>[2x]MTHEEHHAARTLGVGKAIAVLTSGGDAQGMNAAVRAVVRVGIFTGARVFFVHEGYQGLVDGGDHIREATWESVSMMLQLGGTVIGSARCKDFREREGRLRAAHNLVKRGITNLCVIGGDGSLTGADTFRSEWSDLLSDLQKAGKITAEEATRSSYLNIVGLVGSIDNDFCGTDMTIGTDSALHRITEIVDAITTTAQSHQRTFVLEVMGRHCGYLALVTSLSCGADWVFIPECPPDDNWEDHLCRRLSETRTRGSRLNIIIVAEGAIDRNGKPITSEGVKDLVVRRLGYDTRVTVLGHVQRGGTPSAFDRILGSRMGVEAVMALLEGTPDTPACVVSLSGNQAVRLPLMECVQVTKDVTKAMDEKRFDEAMKLRGRSFMNNWEVYKLLAHIRPPAPKSGSYTVAVMNVGAPAAGMNAAVRSTVRIGLIQGNR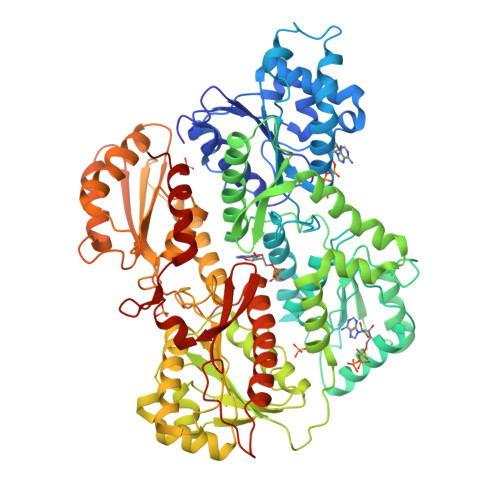VLVVHDGFEGPAKGQIEEAGWSYVGGWTGQGGSKLGSKRTLPKKSFEQISANITKFNIQGLVIIGGFEAYTGGLELMEGRKQFDELCIPFVVIPATVSNNVPGSDFSVGADTALNTICTTCDRIKQSAAGTKRRVFIIETMGGYCGYLATMAGLAAGADAAYIFEEPFTIRDLQANVEHLVQKMKTTVKRGLVLRNEKCNENYTTDFIFNLYSEEGKGIFDSRKNVLGHMQQGGSPTPFDRNFATKMGAKAMNWMAGKIKESYRNGRIFANTPDSGCVLGMRKRALVFQPVTELQNQTDFEHRIPKEQWWLKLRPILKILAKYEIDLDTS> GSHMSAPLPLDELRTFAEVLDRVKAA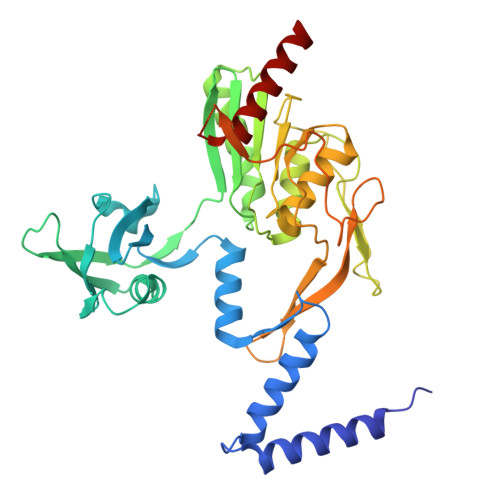YVEPVDDKTLLENAIKGMLSNLDPHSAYLGPEDFAELQESTSGEFGGLGIEVGSEDGFIKVVSPIDDTPAARAGIQPGDLIVQIDGKPTKGQSMTEAVDSMRGKAGSPITLTIVRDGGRPFDVELKRAIIKVKSVKSQVLEPGYAYLRITQFQVNTGEEVVKALNQLRKDNKGRLKGLVLDLRNNPGGVLQSAVEVADAFLTKGLIVYTKGRIANSELRFSADPADPSDKVPLVVLINGGSAAAAEIVAGALQDQKRAILMGTDSFGKGSVQTVLPLNNDRALKLTTALYYTPNGRSIQAQGIVPDIEVGRAKVTQERSSFEGFKEADLQGHLANGNGGADRPTGKRAAPSERPQDSDYQLSQALSLLKGLSVTRGN>ADSDSVLKTVIYSSSGALFMGVWNPSSSGYSDTYSRRIADLVFDSGIPYGIDGVPHPYHCHVVDYKSDVTVPEDAVIFNSTTDTWVAAHAGETAKTYARIECDRPYFHDGHKLSAADVMYSLAWSWEWTTQDGDDDPYYDASEADWSGEYMNTILGIKLVEQTDDRMVFDVYHNHYFPASEIMTAAYVVPFTGTPWQLWYAMSELVAHNPKYSWSESSEDVEQLDQINPSHAQAIKEKLLELKQSKPIPEFLKPYIEDENAATAAYDSIAKFMDEHNHAVIGQGPYYVDEYQPENLFVRIKKFDKWTIPAFAEPEYQVDPYYKTIEVYGIQNEDTAILEVANGHYDILWYPFAAYRFTGLSDEQRANIKLYRSTSAFGDIVWNPVHDQDNPYVITVGDKKYFNPFAVRKVRFAIQYMVNRAYITQNIFQGSAGPMFTPWTSTETGFEYVRPVVDAFGLTEQSDEDLAMKLFEEGMQEAAQELAKMGYELKKGDDGKWYFNGEPVKVVGLGRVEDERKDVATYIVEEVMKKLGFDAEAKIVDRRTASGTVYTSDPSSYQWNFYTEGWVSSSNVKFSTTRIIQ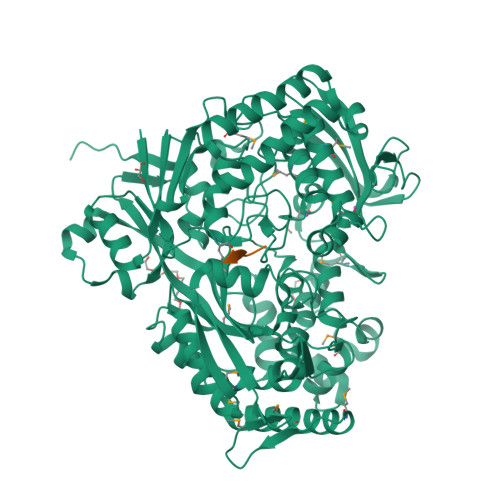YYSSYWYAPGLVGWKWTPENTQRVTMEEVLKFLGNGDIQAGLDSLGLSYYNTVDKIQPLLNWTADDFALVIYSGEANGVKMDSEDKYWDFNRLGTAIGIYEGYRTFLYENWEFYAASKDIEIKLVDPVAGLASDWAIRSARPVVEHHHHHH[4x]> MISIMDRSEIVARENPVITQRVTNLLQTNAPLLFMPIDIHEVRYGAYTLFMYGSLENGYKAEVRIENIPVFFDVQIEFNDTNQLFLKSLLTAENIVYERLETLTQRPVMGYREKEKEFAPYIRIFFKSLYERRKAITYLNNMGYNTAADDTTCYYRMVSRELKLPLTSWIQLQHYSYEPRGLVHRFSVTPEDLVSYQNDGPTDHSIVMAYDIETYSPVKGTVPDPNQANDVVFMICMRIFWIHSTEPLASTCITMAPCKKSSEWTTILCSSEKNLLLSFAEQFSRWAPDICTGFNDSRYDWPFIVEKSMQHGILEEIFNK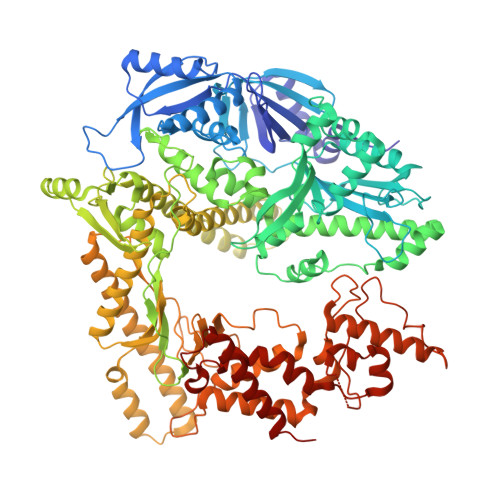MSLFWHQKLDTILKCYYVKEKRVKISAEKSIISSFLHTPGCLPIDVRNMCMQLYPKAEKTSLKAFLENCGLDSKVDLPYHLMWKYYETRDSEKIADVAYYCIIDAQRCQDLLVRHNVIPDRREVGILSYTSLYDCIYYAGGHKVCNMLIAYAIHDEYGRIACSTIARGKREHGKYPGAFVIDPVKGLEQDKPTTGLDFASLYPSLIMAYNFSPEKFVASRDEANSLMAKGESLHYVSFHFNNRLVEGWFVWHNNVPDKMGLYPKVLIDLLNKRTALKQELKKLGEKKECIHESHPGFKELQFRHAMVDAKQKALKIFMNTFYGEAGNNLSPFFLLPLAGGVTSSGQYNLKLVYNFVINKGYGIKYGDTDSLYITCPDSLYTEVTDAYLNSQKTIKHYEQLCHEKVLLSMKAMSTLCAEVNEYLRQDNGTSYLRMAYEEVLFPVCFTGKKKYYGIAHVNTPNFNTKELFIRGIDIIKQGQTKLTKTIGTRIMEESMKLRRPEDHRPPLIEIVKTVLKDAVVNMKQWNFEDFIQTDAWRPDKDNKAVQIFMSRMHARREQLKKHGAAASQFAEPEPGERFSYVIVEKQVQFDIQGHRTDSSRKGDKMEYVSEAKAKNLPIDILFYINNYVLGLCARFINENEEFQPPDNVSNKDEYAQRRAKSYLQKFVQSIHPK>[2x]MGSSHHHHHHSSGLVPRGSHMSGSGSGSGTALTPSYLKDDDGRSLILRGFNTASSAKSAPDGMPQFTEADLAREYADMGTNFVRFLISWRSVEPAPGVYDQQYLDRVEDRVGWYAERGY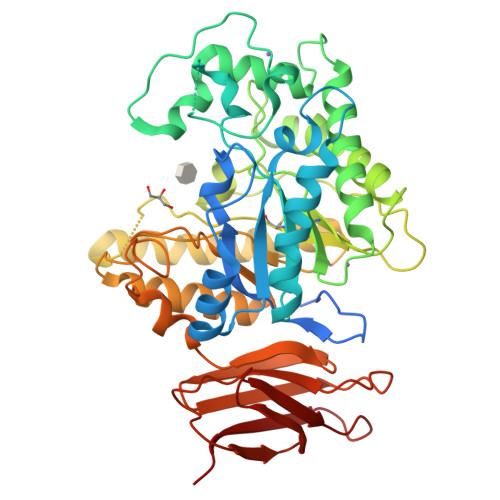KVMLDMHQDVYSGAITPEGNSGNGAGAIGNGAPAWATYMDGLPVEPQPRWELYYIQPGVMRAFDNFWNTTGKHPELVEHYAKAWRAVADRFADNDAVVAYDLMNEPFGGSLQGPAFEAGPLAAMYQRTTDAIRQVDQDTWVCVAPQAIGVNQGLPSGLTKIDDPRAGQQRIAYCPHLYPLPLDIGDGHEGLARTLTDVTIDAWRANTAHTARVLGDVPIILGEFGLDTTLPGARDYIERVYGTAREMGAGVSYWSSDPGPWGPYLPDGTQTLLVDTLNKPYPRAVAGTPTEWSSTSDRLQLTIEPDAAITAPTEIYLPEAGFPGDVHVEGADVVGWDRQSRLLTVRTPADSGNVTVTVTPAA>[4x]MAEYVFSDAPKDSHGNGVKDAVPGKQPEELPP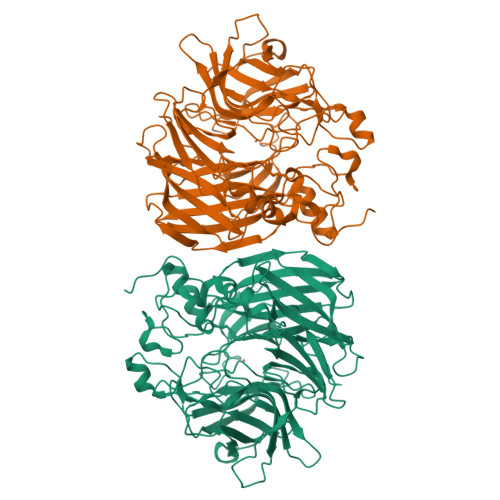APRYFQGENTAGFMRPVRFEGDITNLEVVGEIPKSIEGTFYRVMPEPHLPSFIPNDPWFNGDGNISGFYFKDGHVDLKQRYVRTEKFVREAEARRSLLGKYRNRYTDLVEFKIRSTANTNIVYWRGQLLALKEDSPPYAMDPETLETFGVYDFDGQLPSLTFTAHPKFDPVTREMVCFGYEAKGDGTRDICYYSFGPDGKIAETVWLVSPVCGMIHDFAVTENFVIFPIIPLVCDVERMKQGGDHWQWDYSIPMYIGVLPRRGAQGSDVKWFEAPHGFAGHVANAFEDDKGHIQLQMAYAKDNVFFWWPDANGKGPRPGEVEAHFANFVLDYQSDKLPLAEPTYLVDDDMEFPRIDDRVATRKHKHTFFCIFDRKPGVTDFEFVMPRAGGGAPMSNGLAHLNHETGDIQRYLPGPRKLTGECIFIPRNSEAAEGDGYVMVLLANYEDMCSELAVLDTKDLTNEVALIKLPVRLRPGVHGNWVDKSDVDGHPAPL> XYDYP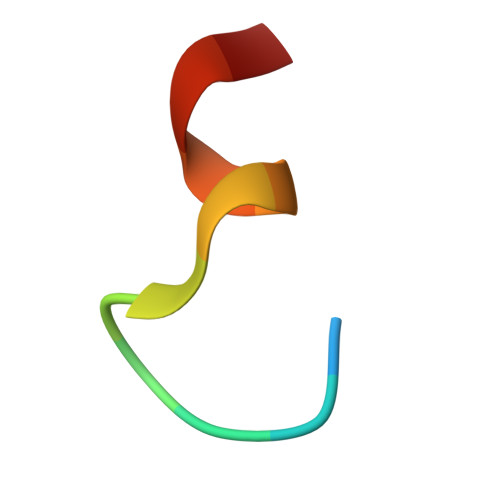GDYCYLYX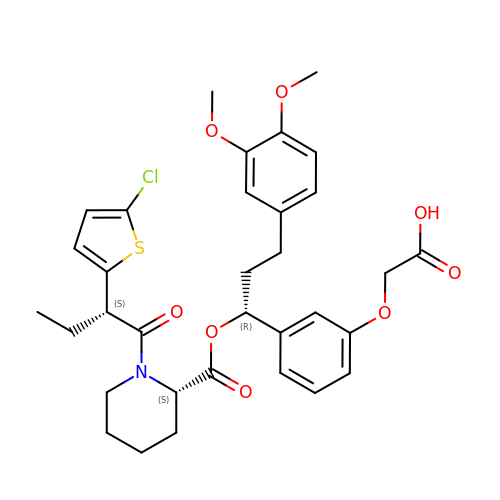2-[3-[(1~{R})-1-[(2~{S})-1-[(2~{S})-2-(5-chloranylthiophen-2-yl)butanoyl]piperidin-2-yl]carbonyloxy-3-(3,4-dimethoxyphenyl)propyl]phenoxy]ethanoic acid | C33 H38 Cl N O8 S | SRIRUOTUARWLRH-UODIDJSMSA-N> GSCQLSQLQCQLAAKEAKLRDLEDSLARERDTSRRLL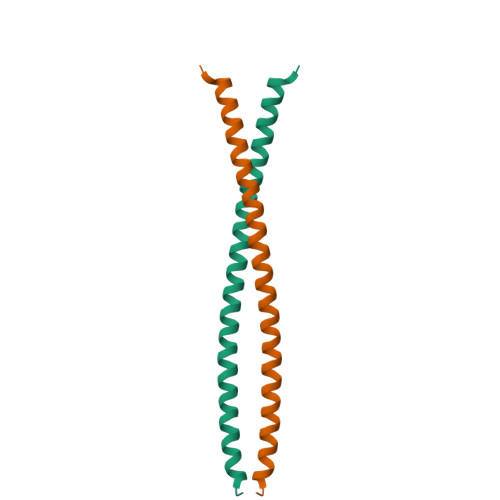AEKEREMAEMRARMQQQLDEYQELLDIKLALDMEIHAYRKLLEGEEERL>SLETVQLRNPPRRQLKKLDEDSLTKQPEEVFDVLEKLGEGSY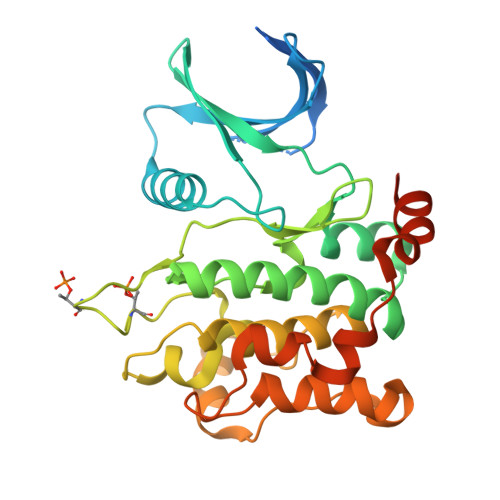GSVYKAIHKETGQIVAIKQVPVESDLQEIIKEISIMQQCDSPHVVKYYGSYFKNTDLWIVMEYCGAGSVSDIIRLRNKTLTEDEIATILQSTLKGLEYLHFMRKIHRDIKAGNILLNTEGHAKLADFGVAGQLTDTMAKRNTVIGTPFWMAPEVIQEIGYNCVADIWSLGITAIEMAEGKPPYADIHPMRAIFMIPTNPPPTFRKPELWSDNFTDFVKQCLVKSPEQRATATQLLQHPFVRSAKGVSILRDLINEAMDVKLKRQESQQREEG[2x]> MGRQWALEDFEIGRPLGKGKFGNVYLAREKQSKFILALKVLFKAQLEKAGVE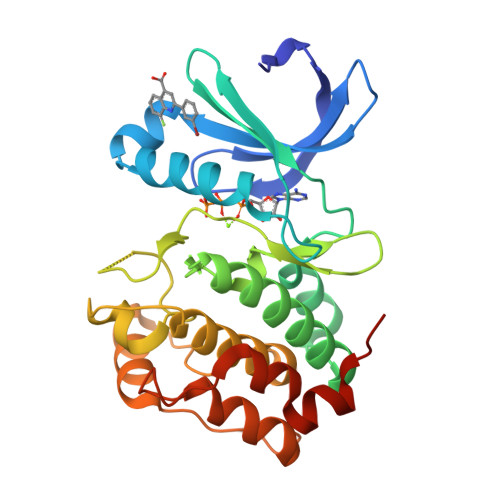HQLRREVEIQSHLRHPNILRLYGYFHDATRVYLILEYAPLGTVYRELQKLSKFDEQRTATYITELANALSYCHSKRVIHRDIKPENLLLGSAGELKIADFGWSVHAPSSRRATLCGTLDYLPPEMIEGRMHDEKVDLWSLGVLCYEFLVGKPPFEANTYQETYKRISRVEFTFPDFVTEGARDLISRLLKHNPSQRPMLREVLEHPWITANSSKPHHHHHH ETHYL-CARBAMIC ACID METHYL ESTER 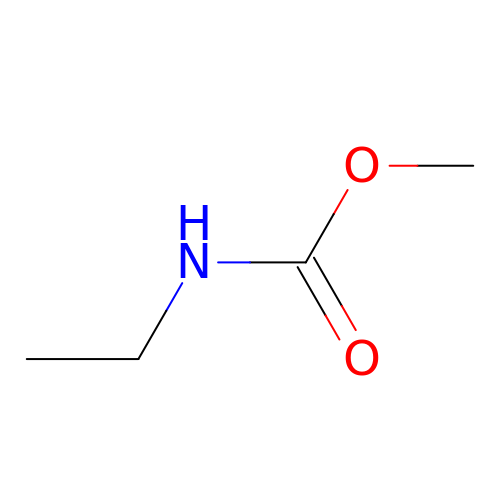| C4 H9 N O2 | AEARPZNULDFPNQ-UHFFFAOYSA-N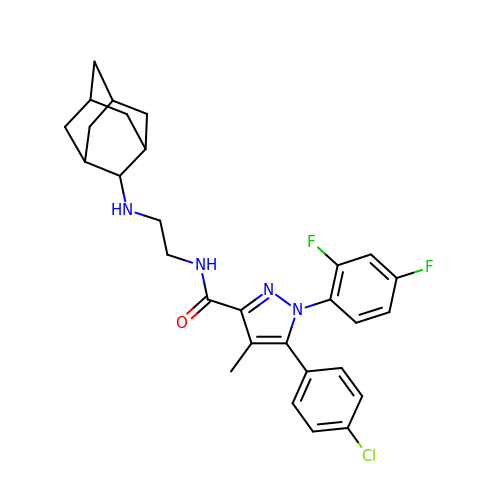N-[2-(2-adamantylamino)ethyl]-1-[2,4-bis(fluoranyl)phenyl]-5-(4-chlorophenyl)-4-methyl-pyrazole-3-carboxamide | C29 H31 Cl F2 N4 O | HCEMTEUNKPHHGT-MXLKCDAXSA-N>AHFPQTPGFSGTLRPLRIEGDILDIEIEGEVPPQLNGTFHRVHPDAQFPPRFEDDQFFNGDGMVSLFRFHDGKIDFRQRYAQTDKWKVERKAGKSLFGAYRNPLTDDASVQGMIRGTANTNVMVHAGKLYAMKEDSPCLIMDPLTLETEGYTNFDGKLQSQTFCAHPKIDPVTGNLCAFAYGAKGLMTLDMAYIEISPTGKLLKEIPFQNPYYCMMHDFGVTEDYAVFAVMPLLSSWDRLEQRLPFFGFDTTLPCYLGILPRNGDARDLRWFKTGNCFVGHVMNAFNDGTK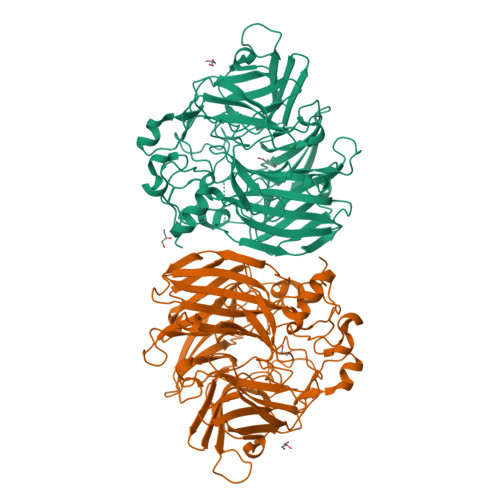VHIDMPVSRNNSFPFFDVHGAPFDPVAGQGFLTRWTVDMASNGDSFEKTERLFDRPDEFPRIDERYATRAYRHGWMLILDTEKPYEAPGGAFYALTNTLGHIDLATGKSSSWWAGPRCAIQEPCFIPRSPDAPEGDGYVIALVDDHVANYSDLAIFDAQHVDQGPIARAKLPVRIRQGLHGNWADASRLAA[2x]>GAPSNIAGMIVFLDPGHNGANDASIGRQVPTGRGGTKNCQESGTATDDGYPEHSFTWDTTLRVRAALTALGVRTAMSRGNDNALGPCVDERAAMANSLRPHAIVSIHADGGPPTGRGFHVLYSSPPLNAAQSGPSVQFAKVMRDQLAASGIPPATYIGQGGLNPRSDIAGLNLAQFPSVLVECGNMKNPVDSALMKSPEGRQKYADAIVRGIAGFLGSQSQAAAAVSP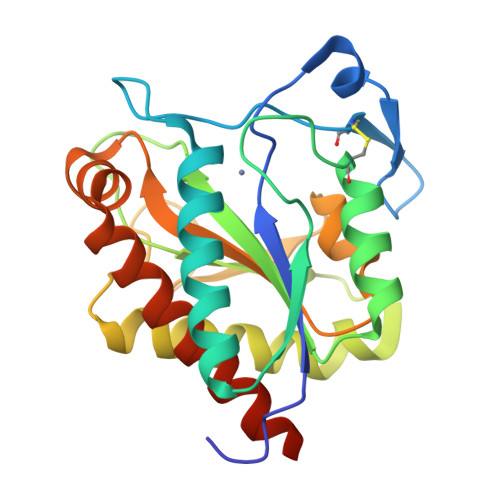VR[2x]[[(2~{R},3~{S},5~{R})-5-[4-[(4~{R})-4,5-bis(oxidanyl)pent-1-ynyl]-2-nitro-pyrrol-1-yl]-3-oxidanyl-oxolan-2-yl]methoxy-oxidanyl-phosphoryl] 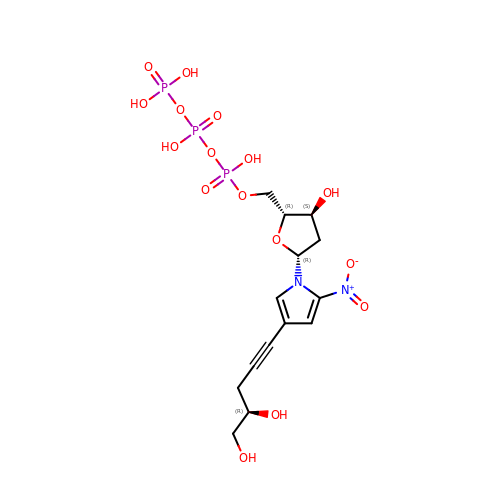phosphono hydrogen phosphate | C14 H21 N2 O16 P3 | JIVPAQSXWIKFCI-GFQSEFKGSA-N> MRALLLTTLAVLAVGINAAESDSRARVVCYFSNWAVYRPGVGRYGIEDIPVDMCTHIIYSFIGVTEDTQQVLIIDPELDVDKNGFKNFTSLRSKHPGVKFTVAVGGWAEGGSKYSKMVAAKSTRMAFVRSVVDFLNKYNFDGLDLDWEYPGAADRGGSFSDKDKFLYLVQELRRAFIREGKGWELTAAVPLANFRLMEGYHVPELCQELDAIHVMSYDLRGNWAGFADVHSPLYKRPHDQWAYEKLNVNDGLQLWEDKGCPTNKLVVGIPFYGRSFTLSSGNNNYNLGTYINKEAGGGDPAPYTNATGFWAYYEICTEVDTADSKWTKKWDEHGKCPYAYKGTQWVGYEDPRSVEIKMNWIKEKGYLGAMTWAIDMDDFQGLCGEKNILIKLLHKHMSAYTVPPPRSGNTTPTPEWARPPSTPSDPSEGDPIPTTTTSKPATSKPSTTSQPATTSRPEPKPTTSLPTPAPTASTTEEEAQQPEVELPAENEIGNSDKICTSEEDYIPDKKQCDKYWRCVNGEGMQFKCQPGTVFNVKLNVCDWPENADRHDCQL

The glycosyl hydrolase family 18 (GH18) chitinases (EC 3.2.1.14) are enzymes that hydrolyze chitin, a β-1,4-linked N-­acetylglucosamine (GlcNAc) linear polymer, into chito­oligosaccharides. Among the eight groups of insect chitinases, group I chitinases have been enzymatically well characterized and have been shown to function in a chitin-degradation process that is closely associated with insect moulting. Our previous work reported on the group I insect chitinase OfChtI (previously called OfCht5) from Ostrinia furnacalis, a species of moth that is the most destructive insect affecting corn production. OfChtI is highly active in the hydrolysis of chitooligosaccharides, colloidal chitin and α-chitin, and exhibits kinetic properties that differ from those of bacterial and plant chitinases.

Thus, the truncated form of OfChtI (OfChtI-CAD; residues 19–407) was cloned, expressed and purified for crystallization. OfChtI-CAD crystals were obtained by vapour diffusion and the structure was determined by X-ray diffraction. The crystals belonged to space group P65 and the structure was solved at a resolution of 1.7 Å. The final solved structure contained residues Arg24–Arg406 with two N-GlcNAc residues at the N-glycosylation sites Asn87 and Asn305. Like most reported chitinases, OfChtI-CAD folds into two distinct domains: a core domain and an insertion domain (CID). The chitinase signature motif ‘DxDxE’ (Asp144–Glu148) is located in the loop between strand β4 and helix α4. According to the catalytic mechanism, the glutamate residue Glu148 is the catalytic acid/base, the aspartic acid residue Asp146 is critical for stabilizing the enzyme–substrate intermediate, and Asp144 appears to be crucial for keeping Asp146 protonated. A long substrate-binding cleft was observed on the surface of OfChtI-CAD and its volume was estimated to be 1628 Å3, with a surface area of 999 Å2, using the CASTp software. The cleft is composed of a set of aligned aromatic residues that includes Trp34, Tyr37, Phe61, Trp107, Phe194, Trp223, Trp241, Tyr243 and Trp372. Surprisingly, a unique flat plane characterized by four aromatic residues, Phe159, Phe194, Trp241 and Tyr290, was observed on the surface of OfChtI-CAD.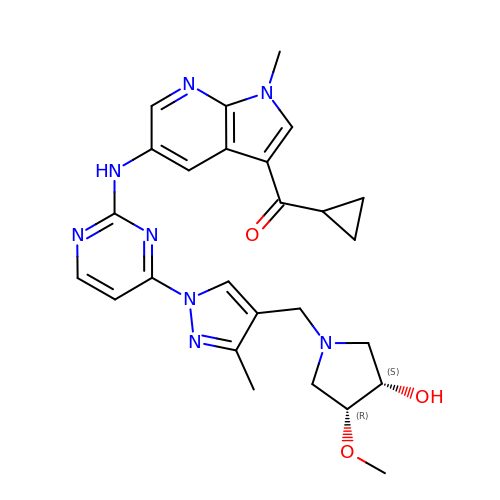cyclopropyl-[5-[[4-[4-[[(3~{R},4~{S})-3-methoxy-4-oxidanyl-pyrrolidin-1-yl]methyl]-3-methyl-pyrazol-1-yl]pyrimidin-2-yl]amino]-1-methyl-pyrrolo[2,3-b]pyridin-3-yl]methanone | C26 H30 N8 O3 | XJLACMXDBBMNAD-FCHUYYIVSA-N7-CL-D-TRYPTOPHAN | C11 H11 Cl N2 O2 | 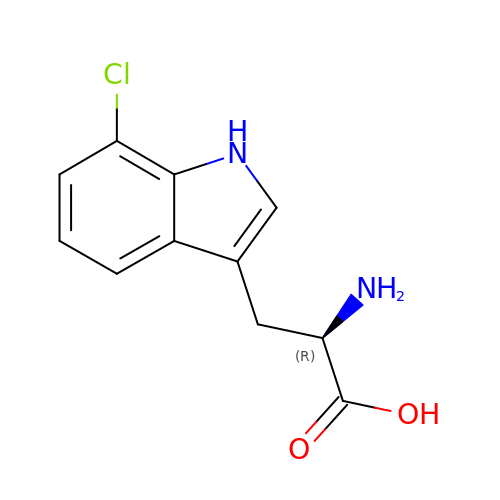DMQFGLHRDFQKNR-SECBINFHSA-N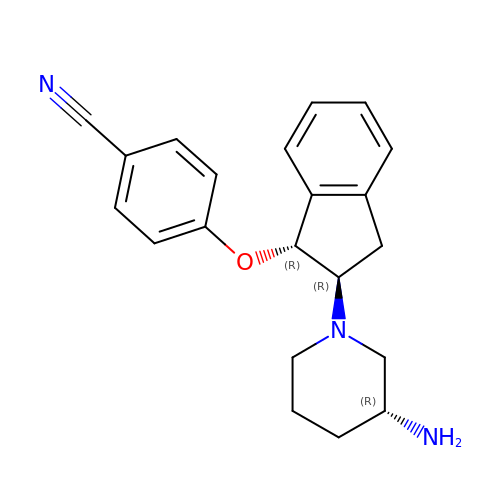4-({(1R,2R)-2-[(3R)-3-aminopiperidin-1-yl]-2,3-dihydro-1H-inden-1-yl}oxy)benzonitrile | C21 H23 N3 O | IVKKIBLLVHIRDV-DUXKGJEZSA-N>MVARPKSEDKKQALLEAATQAIAQSGIAASTAVIARNAGVA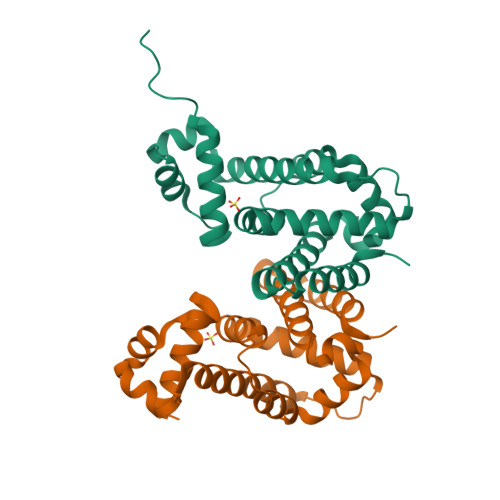EGTLFRYFATKDELINTLYLHLKQDLCQSMIMELDRSITDAKMMTRFIWNSYISWGLNHPARHRAIRQLAVSEKLTKETEQRADDMFPELRDLCHRSVLMVFMSDEYRAFGDGLFLALAETTMDFAARDPARAGEYIALGFEAMWRALTREEQ[2x]>[2x]SNAMTQQDFRTKVDN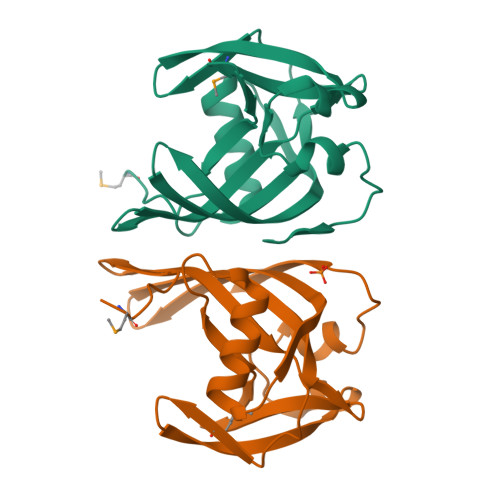TVFGVRATALIVQNHKLLVTKDKGKYYTIGGAIQVNESTEDAVVREVKEELGVKAQAGQLAFVVENRFEVDGVSYHNIEFHYLVDLLEDAPLTMQEDEKRQPCEWIDLDKLQNIQLVPVFLKTALPDWEGQLRHIHLEE>[4x]MRIPLVGKDSIESKDIGFTLIHEHLRVFSEAVRQQWPHLYNEDEEFRNAVNEVKRAMQFGVKTIVDPTVMGLGRDIRFMEKVVKATGINLVAGTGIYIYIDLPFYFLNRSIDEIADLFIHDIKEGIQGTLNKAGFVKIAADEPGITKDVEKVIRAAAIANKETKVPIITHSNAHNNTGLEQQRILTEEGVDPGKILIGHLGDTDNIDYIKKIADKGSFIGLDRYGLDLFLPVDKR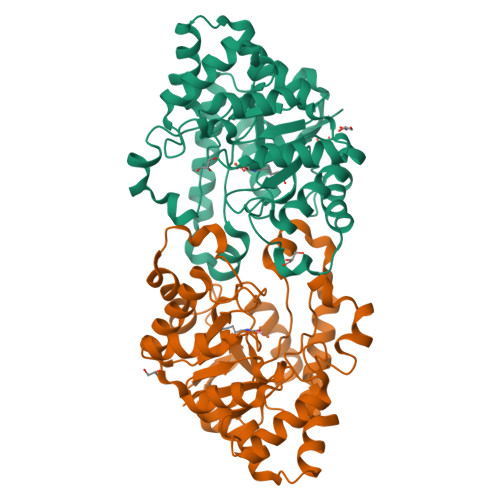NETTLRLIKDGYSDKIMISHDYCCTIDFGTAKPEYKPKLAPRWSITLIFEDTIPFLKRNGVNEEVIATIFKENPKKFFS>[2x]GSDELKWNKGYSLPNLLE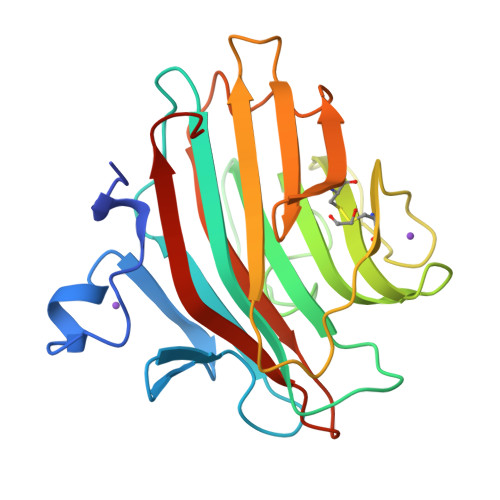VTDQQKELSQWTLGDKVKLEEGRFVLTPGKNTKGSLWLKPEYSIKDAMTIEWTFRSFGFRGSTKGGLAFWLKQGNEGDSTELFGGSSKKFNGLMILLRLDDKLGESVTAYLNDGTKDLDIESSPYFASCLFQYQDSMVPSTLRLTYNPLDNHLLKLQMDNRVCFQTRKVKFMGSSPFRIGTSAINDASKESFEILKMKLYDGVIEDSL>APQLHHHHHHDLYENLYFQGKLDPASKSRSCGEVRQIYGAKGFSLSDVPQAEISGEHLRICPQGYTCCTSEMEENLANRSHAELETALRDSSRVLQAMLATQLRSFDDHFQHLLNDSERTLQATFPGAFGELYTQNARAFRDLYSELRLYYRGANLHLEETLAEFWARLLERLFKQLHPQLLLPDDYLDCLGKQAEALRPFGEAPRELRLRATRAFVAARSFVQGLGVASDVVRKVAQVPLGPECSRAVMKLVYCAHCLGVPGARPCPDYCRNVLKGCLANQADLDAEWRNLLDSMVLITDKFWGTSGVESVIGSVHTWLAEAINALQDNRDTLTAKVIQGCGNPKVNPQGPGPEEKRRRGKLAPRERPPSGTLEKLVSEAKAQLRDVQDFWISLPGTLCSEKMALSTASDDRCWNGMARGRYLPEVMGDGLANQINNPEVEVDITKPDMTIRQQIMQLKIMTNRLRSAYNG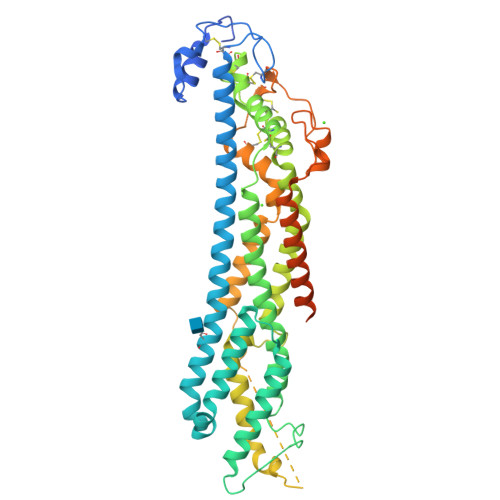NDVDFQDASDDGAGAGAGDGCLDDLCSRKVSRKSSSSRTPLTHALPGLSEQEGQ[4x]> MVMLSDPNLVLFYVKNPAKSEEFYKNLLDTQPIESSPTFAMFVMKTGLRLGLWAQEEIEPKAHQTGGGMELSFQVNSNEMVDEIHRQWSDKEISIIQPPTQMDFGYTFVGVDPDEHRLRIFCLKRTAE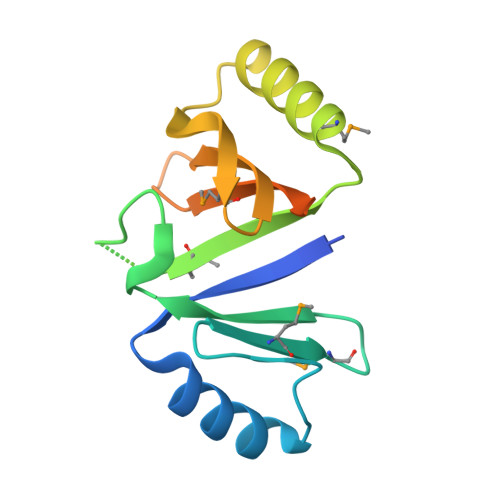NLYFQSHHHHHHWSHPQFEK> RKKQDPPVTHDLRVSLEEIYSGCTKKMKISHKRLNPDGKSIRNEDKILTIEVKKGWKEGTKITFPKEGDQTSNNIPADIVFVLKDKPHNIFKRDGSDVIYPARISLREALCGCTVNVPTLDGRTIPVVFKDVIRPGMRRKVPGEGLPLPKTPEKRGDLIIEFEVIFPERIPQTSRTVLEQVLPI;> SGPQIKELTDEEAERLQLEIDQK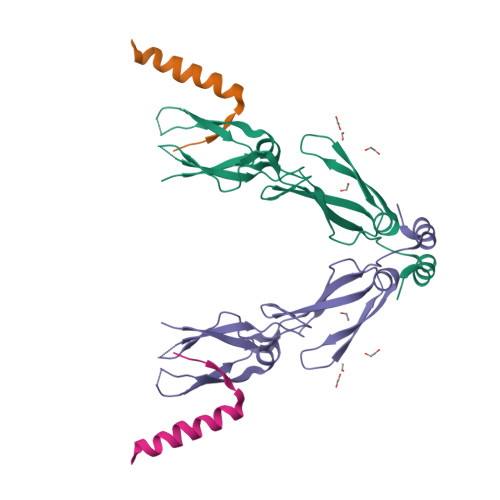KDAENHEAQLKNGSLDSPG Centrioles have proximal-distal polarity and a 9-fold radial symmetry imparted by a likewise symmetrical central scaffold, the cartwheel. The spindle assembly abnormal protein 6 (SAS-6) self-assembles into 9-fold radially symmetric ring-shaped oligomers that stack via an unknown mechanism to form the cartwheel. SAS-6 proteins comprise a globular “head” domain at their N-terminus followed by a long coiled coil that mediates stable protein homo-dimerization (Keller et al., 2014), and a disordered C-terminal extension. The characteristic shape of the SAS-6 ring led to the proposal that the protein head domains comprise the central “hub” of the centriolar cartwheel, with SAS-6 coiled coils forming the cartwheel “spokes” (Cottee et al., 2015; Kitagawa et al., 2011; van Breugel et al., 2011; van Breugel et al., 2014; Yoshiba et al., 2019).

Recombinantly produced fragments of the corresponding coiled-coil domains were folded, as judged by thermal denaturation experiments monitored by circular dichroism (CD) spectroscopy, and formed dimers in solution size exclusion chromatography–multiangle light scattering (SEC-MALS) assays. We succeeded in crystalizing a fragment of the coiled-coil domain from each species, with different boundaries, but spanning approximately the middle one-third of this protein region (henceforth, CrSAS-6_CCMiddle, DrSAS-6_CCMiddle, and HsSAS-6_CCMiddle; see Figure S2A for the protein sequence alignment, Table 1 for a list of recombinant protein constructs, and Figure S1A for SDS-PAGE analysis of these constructs). As the HsSAS-6_CCMiddle and DrSAS-6_CCMiddle fragments did not originally include methionine residues, one or two amino acids, respectively, were mutated to methionine to allow SeMet incorporation. All three SAS-6 structures revealed two-stranded parallel coiled-coil domains as analyzed by SOCKET, in agreement with the predicted nature of this protein section. The HsSAS-6_CCMiddle coiled coil is distorted compared with a canonical CC structure at a region N-terminal to the site of SeMet incorporation (indicated). Only parallel associations between coiled-coil domains are compatible with the stacking of SAS-6 rings into a continuous cartwheel, whereas antiparallel coiled-coil interactions would lead to horizontal displacement of SAS-6 rings, a distribution incompatible with a stacked rings configuration. Both the HsSAS-6_CCMiddle and DrSAS-6_CCMiddle crystal structures revealed primarily antiparallel associations between their coiled coils, with only much smaller parallel associations between coiled-coil copies, which were offset by approximately one-half length or the full length of the crystallographic c-axis, respectively.

>GPSQELTNEKEKALQAQVQYQQQHEQQKKDLEILHQQNIHQLQNRMSELEAANKDLTERKYKGDSTIRELKAKLSGVEEELQRTKQEVLSLRRENSTLDVECHE[6x]>MGHHHHHHSGMKIAILGAMSEEITPLLETLKDYTKIEHANNTYYFAKYKDHELVLAYSKIGKVNSTLSASVMIEKFGAQVLLFTGVAGAFNPELEIGDLLYATKLAQYDLDITAFGHPLGFVPGNEIFIKTDEKLNNLALEVAKELNIKLRAGIIATGDEFICDEA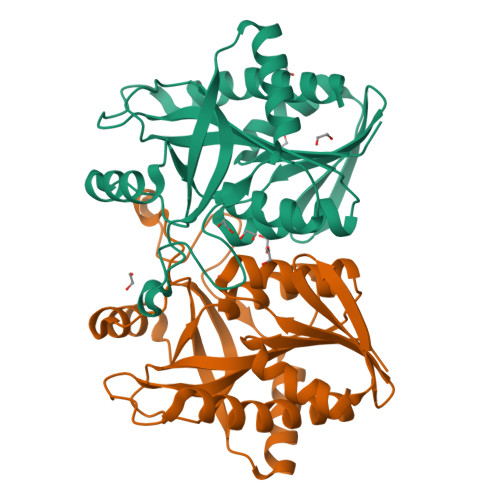KKAKIREIFNADACEMEGASVALVCDALKVPCFILRAMSDKAGEKAEFDFDEFVINSAKISANFVLKMCEKL[2x]>MAKSDVKLLGAWPSPYVMRARITLNVKSVDYELLEETLGSKSDLLLKSNPVHKKIPVLIHNDKPICESLIIVHYIDEFWSSGPSILPSDPYDRAIARFWAAYLDEKWYPSLKGIASAQGEEAKKAAVDQVG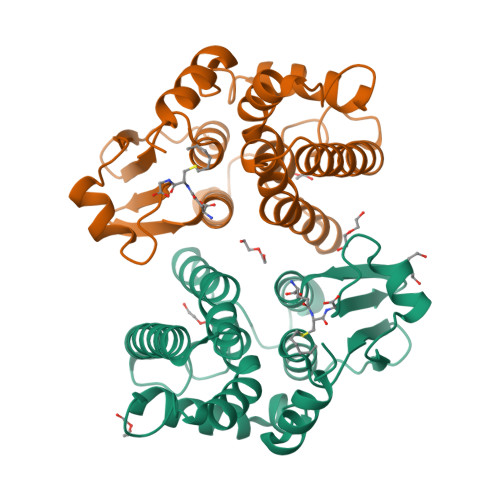ESLALIEDTYVKLSKGKPFFGGEKIGYLDIAFGCFLGWLRVTEKTSGVKFLNEAKTPHLAKWAVRFCADPAVKDVMPETEKLAEFAKLLAKFRAGPPK[2x]> MEEDIACVKDLVSKYLANNERLSRQKLAFLVQTEPRMLLMEGLKLLSLCIEVDSCNANGCEHNSEDKSVERILHDHGVLTPSLCFVVPDGYKLTGNVLILLECFVRSSPANFEQKYVEDFKKLEQLKEDLKSVDINLIPLIDGRTSFYNEQIPDWVNDKLRDTLFSLLKYAQESNSLFEESEYSRLCESLSMTSGRLSGVESLNALLDNRSNHYEEVIASCHQGINNKLTAHEVKLQIEEEYQVFRNRLRKGEIEGQFLKVEKNQLLNEFNNL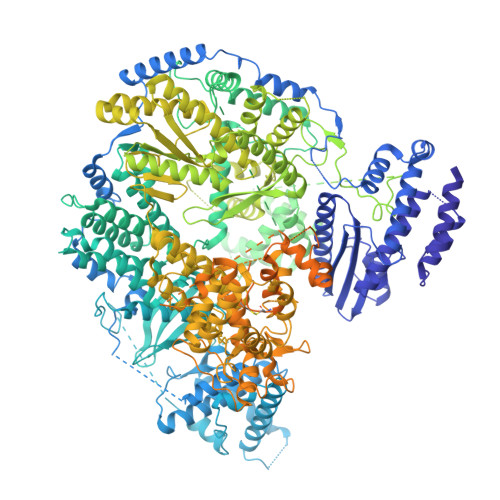YADKVAEKDSVEHLTHQFKRASPILRFLYANISKGDNGEGNLIIGECQMQCWRSFLNKVKSMRILNTRRKLLLIFDALILLASKHDQVRKKPLRGWLGTCFVSVNDRLVSLESTKKDLKKWVERRQQVERSRTMQSFQCPSKNQILNSIFQKTISKATTALRDVGISVDHYKIDMEVICPDGYDLIMDFDVSGVTPTISYQRSEEEAFPYIMGDVDLLKTTDLERLSSLSLALVNSMKTSSTVKLRQNEFGPARYQVVKCKEAYCQEFSLGETEFQLIYQKTGECSKCYAINDNRVGEVCSFYADPKRYFPAIFSAEVLQTTVSTMISWIEDCNELEEQLDKIRSLTKMILILILAHPSKRSQKLLQNLRYFIMAYVSDYYHKDLIDKVREELITDVEFLLYRLLRTLMGLVLSEDVKSMMTNRFKFILNISYMCHFITKETPDRLTDQIKCFEKFLEPKVKFGHVSINPADTATEEELDDMVYNAKKFLSKGGCTSAKGPSYKKPGVSKKYLSLLTSSFNNGSLFKEREVKKEIKDPLITSGCATALDLASNKSVVVNKYTDGSRVLNYDFNKLTALAVSQLTEVFSRKGKHLLNKQDYEYKVQQAMSNLVLGSKQHKGDADEADLDEILLDGGASTYFNQLKETVEKIVDQYREPVKMGSGSNDGDQPSINDLDEIVSNKFYIRLIKGELSNHMVEDFDHDVLPDKFYEEFCDAVYENSKLKEKYFYCGHMSQCPIGELTKAVSTRTYLDHEYFQCFKSILLIMNANALMGKYTHYKSRNLNFKFDMGKLSDDARISERESNSEALSKALSLTNCTTAMLKNLCFYSQESPQSYNSVGPDTGRLKFSLSYKEQVGGNRELYIGDLRTKMFTRLIEDYFEALSSQLSGSCLNNEKEFENAILSMKLNVSMAHVSYSMDHSKWGPMMCPFLFLTVLQNLIFLSKDLQADIKGRDYLSTLLMWHMHKMVEIPFNVVSAMMKSFIKAQLGLRKKTKQSITEDFFYSNFQIGVVPSHISSILDMGQGILHNTSDFYALITERFINYAISCVCGGTIDAYTSSDDQISLFDQTLTELLHRDPEEFRALMEFHYYMSDQLNKFVSPKSVIGRFVAEFKSRFFVWGDEVPLLTKFVAAALHNIKCKEPHQLAETIDTIVDQSVANGVPVHLCNLIQIRTLSLLQYARYPIDPFLLNCETDVRDWVDGNRSYRIMRQIEGLIPDACSKIRSMLRRLYNRLKTGQLHEEFTTNYLSSEHLSSLKNLCELLGVEPPSESDLEYSWLNLAAHHPLRMVLRQKIIYSGAVNLDDEKIPTIVKTIQNKLSSTFTRGAQKLLSEAINKSAFQSSIASGFVGLCRTLGSKCVRGPNKENLYIKSIQSLITGTQGIELLTNSIGVQYWRVPLGLRNKSESVVSYFRPLLWDYMCISLSTAIELGAWVLGDPKTTKALDFFKHNPCDYFPLKPTASKLLEDRVGLNHIIHSLRRLYPSVFEKHILPFMSDLASTKMKWSPRIKFLDLCVALDVNCEALSLVSHIVKWKREEHYIVLSSELRFSHTRTHEPMVEERVVSTSDAVDNFMRQIYFESYVRPFVATTRTLGSFTWFPHRTSIPEGEGLHRLGPFSSFVEKVIHKGVERPMFKHDLMMGYAWIDFDIEPARFNQNQLIASGLVDSKFDSLEDFFDAVASLPTGSAKLSQTVRFRIKSQDASFRESFAIHLDYIGSMNQQAKYLVHDVTAMYSGAVSPCVLSDCWRLVLSGPTFKGKPVWYVDTEVINEFLVDTNQLGHVTPVEVVVDMEKLQFAEYDFMLVGPCAEPVPLVVRRGGLWECEKKLASFTPVIQDQDLEMFVREVGDTSSDLLIRALSDMITDRLGLRMQWSGVDIVSTLRAAAPGNAEVLSAVLEVVDNWVEFKGYALCYSKSRGRVMVQSSSGKLRLKGRTCEELTEGGEHVEDIE>[2x]SNAIESRRAVVRAWGNQSIEEADPEIHEFMEKEKQRQFRGIELIASENFVCRAVMEALGSHLTNKYSEGMPGARYYTGNQYIDQIEILCQERALAAFGLNHEKWGVNVQPYSCTSANFAVFTGLLMPGERIMGLDSPSGGHMSHGYYTPGGKKVSGASIFFESFPYKVDPRTGYIDYDKLEEKALDYRPKI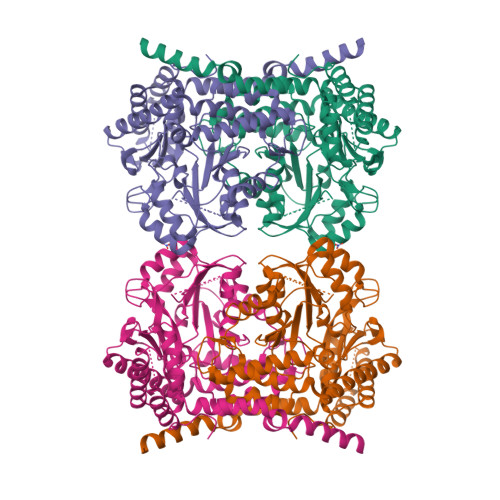LICGGSSYPRDWEFPRFRHIADKCGAVLMFDMAQISGLVAAKESPNPFDYCDIVTSTTHKSLRGPRGGIIFYKRGLKPKKQSINLNHCESNIQYDFEEKINFSVFPSLQGGPHNNHIAALAIALKQAASPEYKLYMRQVKKNAKALASALISRKCKLITGGTDNHLLLWDLTPLGLTGKVYEKVCEMCHITVNKVAIFSENGVISPGGVRIGSPAMTSRGCLEPEFETMADFLYRAAQIASAAQREHGKLQKEPLKSIYHCKEIADLRNQVEAFATQFAMPAFDM CHS is the first committed enzyme in flavonoid synthesis and belongs to the superfamily of type three polyketide synthases. Then, chalcone synthase (CHS) condenses one coumaroyl-CoA and three malonyl-CoA to form naringenin chalcone, which is subsequently converted to the (2S)-naringenin by chalcone isomerase (CHI). We determined the crystal structure of HvCHS in complex with CoA, CoA and naringenin, and CoA and eriodictyol.

The initial crystallization experiments with purified HvCHS yielded high-quality crystals that diffracted to 1.7 Å. In the refined structure, we observed an additional electron density in the substrate-binding cleft separating the N- and C-terminal domains, which we interpreted as CoA. All three HvCHS structures are highly congruent, even in residues lining the active site. The only difference can be seen in the β-sheet and loop from L269 to D272. Based on the electron density map, this loop appears to adopt two distinct conformations in all three crystal structures. However, while in the CoA-bound and the CoA/eriodictoyl-bound structures, the “in”-conformation has much higher occupancy and was therefore chosen for the final model, the “out”-conformation is dominant in the naringenin-bound structure. When mapping the active site residues known from the well-studied MsCHS enzyme, and our HvCHS structures, it becomes apparent that the residues in the substrate-binding channel and especially the cinnamoyl-binding pocket are highly conserved. The only differences are residue 199 in HvCHS, where the conserved threonine is replaced by an alanine, and residue 267 in HvCHS, where the conserved phenylalanine is replaced by an isoleucine.

>[2x]MGSSHHHHHHSQDPNSSSMAAVRLKEVRMAQRAEGLATVLAIGTAVPANCVYQATYPDYYFRVTKSEHLADLKEKFQRMCDKSMIRKRHMHLTEEILIKNPKICAHMETSLDARHAIALVEVPKLGQGAAEKAIKEWGQPLSKITHLVFCTTSGVDMPGADYQLTKLLGLSPTVKRLMMYQQGCFGGATVLRLAKDIAENNRGARVLVVCSEITAMAFRGPCKSHLDSLVGHALFGDGAAAAIIGADPDQLDEQPVFQLVSASQTILPESEGAIDGHLTEAGLTIHLLKDVPGLISENIEQALEDAFEPLGIHNWNSIFWIAHPGGPAILDRVEDRVGLDKKRMRASREVLSEYGNMSSASVLFVLDVMRKSSAKDGLATTGEGKDWGVLFGFGPGLTVETLVLHSVPVPVPTAASA> GENFMDIECFMVLNPSQQLAIAVLSLTLGTFTVLENLLVLCVILHSRSLRCRPSYHFIGSLAVADLLGSVIFVYSFIDFHVFHRKDSRNVFLFKLGGVTASFTASVGSLFLAAIDRYISIHRPLAYKRIVTRPKAVVAFCLMWTIAIVIAVLPLLGWNCEKLQSVCSDIFPHIDKTYLMFWIGVVSVLLLFIVYAYMYILWKAHSHAVAKALIVYGSTTGNTEYTAETIARELADAGYEVDSRDAASVEAGGLFEG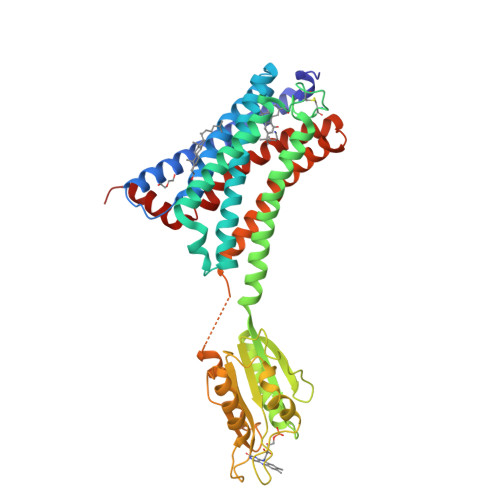FDLVLLGCSTWGDDSIELQDDFIPLFDSLEETGAQGRKVACFGCGDSSWEYFCGAVDAIEEKLKNLGAEIVQDGLRIDGDPRAARDDIVGWAHDVRGAIPDQARMDIELAKTLVLILVVLIICWGPLLAIMVYDVFGKMNKLIKTVFAFCSMLCLLNSTVNPIIYALRSKDLRHAFRSMFPS> PMIDLYTAATPNGHKVSIALEEMGLPYTVHALSFDKKEQKAPEFLRINPNGR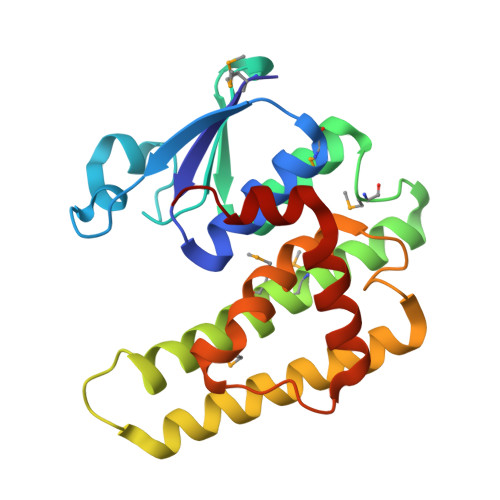IPAIVDRSNDDFAVFESGAILVYLAEKTGQLMPTDVKGRSRVIQWLMFQMGGVGPMQGQANVFFRYFPEKLQGAIDRYQHETRRLYEVLDGRLGEAEYLAGDYSIADIATYPWVRIHDWSGVAVDGLDNLQRWIAALEARPAVQRGLLVPR>STAGKVIKCKAAVLWEEKKPFSIEEVEVAPPKAHEVRIKMVATGICRSDDHVVSGTLVTPLPVIAGHEAAGIVESIGEGVTTVRPGDKVIPLFTPQCGKCRVCKHPEGNFCLKNDLSMPRGTMQDGTSRFTCRGKPIHHFLGTSTFSQYTVVDEISVAKIDAASPLEKVCLIGCGFSTGYGSAVKVAKVTQGSTCAVFGLGGVGLSVIMGCKAAGAARIVGVDINKDKFAKAKEVGATECVNPQDYKKPIQEVLTEMSNGGVDFSFEVIGRLDTMVTALSCCQEAYGVSVIVGVPPDSQNLSMNPMLLLSGRTWKGAIFGGFKSKDSVPKLVADFMAKKFALDPLITH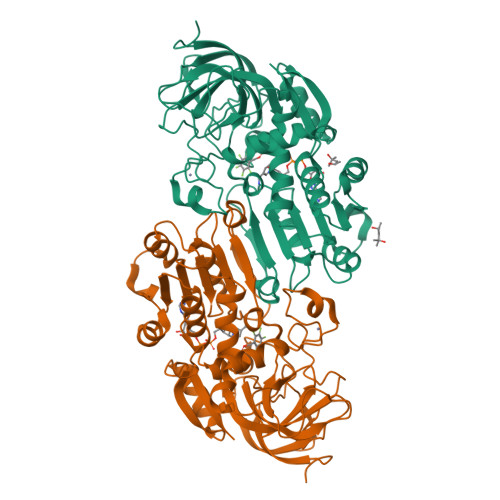VLPFEKINEGFDLLRSGESIRTILTF[2x]> MELADVGAAASSQGVHDQVLPTPNASSRVIVHVDLDCFYAQVEMISNPELKDKPLGVQQKYLVVTCNYEARKLGVKKLMNVRDAKEKCPQLVLVNGEDLTRYREMSYKVTELLEEFSPVVERLGFDENFVDLTEMVEKRL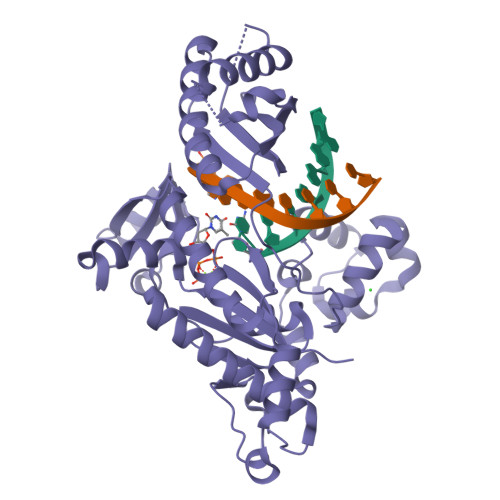QQLQSDELSAVTVSGHVYNNQSINLLDVLHIRLLVGSQIAAEMREAMYNQLGLTGCAGVASNKLLAKLVSGVFKPNQQTVLLPESCQHLIHSLNHIKEIPGIGYKTAKCLEALGINSVRDLQTFSPKILEKELGISVAQRIQKLSFGEDNSPVILSGPPQSFSEEDSFKKCSSEVEAKNKIEELLASLLNRVCQDGRKPHTVRLIIRRYSSEKHYGRESRQCPIPSHVIQKLGTGNYDVMTPMVDILMKLFRNMVNVKMPFHLTLLSVCFCNLKALNTAK> MKLSLTKVVNGCRLGKIKNLGKTGDHTMDIPGCLLYTKTGSAPHLTHHTLHNIHGVPAMAQLTLSSLAEHHEVLTEYKEGVGKFIGMPESLLYCSLHDPVSPCPAGYVTNKSVSVWSVAGRVEMTVSKFMAIQKALQPDWFQCLSDGEVSCKEATSIKRVRKSVDRSLLF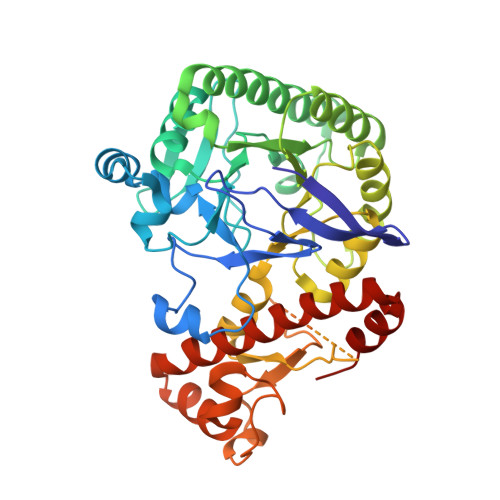LDNCLRLQEESEVLQKSVIIGVIEGGDVMEERLRSARETAKRPVGGFLLDGFQGNPTTLEARLRLLSSVTAELPEDKPRLISGVSRPDEVLECIERGVDLFESFFPYQVTERGCALTFSFDYQPNPEETLLQQNGTQEEIKCMDQIKKIETTGCNQEITSFEINLKEKKYQEDFNPLVRGCSCYCCKNHTRAYIHHLLVTNELLAGVLLMMHNFEHYFGFFHYIREALKSDKLAQLKELIHRQAS> FTLIELMIVIAIVGILAAVALPAYQDYTARAQVSEAILLAEGQKSAVTEYYLNHGKWPENNTSAGVASSPTDIKGKYVKEVEV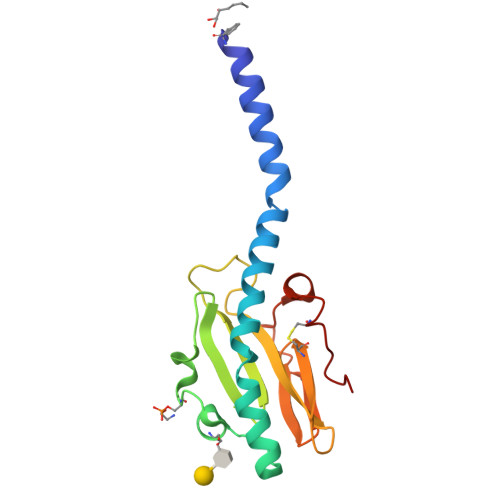KNGVVTATMLSSGVNNEIKGKKLSLWARRENGSVKWFCGQPVTRTDDDTVADAKDGKEIDTKHLPSTCRDNFDAK>[2x]SNAMSAVMTPAGFTDYKVADITLAAWGRRELIIAESEMPALMGLRRKYAGQQPLKGAKILGCIHMTIQTGVLIETLVALGAEVRWSSCNIFSTQDQAAAAIAAAGIPVFAWKGETEEEYEWCIEQTILKDGQPWDANMVLDDGGDLTEILHKKYPQMLERIHGITEETTTGVHRLLDMLKNGTLKVPAINVNDSVTKSKNDNKYGCRHSLNDAIKRGTDHLLSGKQALVIGYGDVGKGSSQSLRQEGMIVKVAEVDPICAMQACMDGFEVVSPYKNGINDGTEASIDAALLGKIDLIVTTTGNVNVCDANMLKALKKRAVVCNIGHFDNEIDTAFMRKNWAWEEVKPQVHKIHRTGKDGFDAHNDDYLILLAEGRLVNLGNATGHPSRIMDGSFANQVLAQIHLFEQKYADLPAAEKAKRLSVEVLPKKLDEEVALEMVKGFGGVVTQLTPKQAEYIGVSVEGPFKPDTYRY

By hydrolyzing SAH to adenosine (Ado) and L-homocysteine (Hcy), the enzyme SAHase (SAH hydrolase) serves as an important regulator of SAM-dependent methylation through the control of the SAM:SAH ratio, and is an indicator of the biological methylation activity of the cell. SAHases are usually active as homotetramers. The protomer has a three-domain fold, with two prominent domains, the substrate- and cofactor-binding domains, separated by a deep crevice. A small C-terminal dimerization domain locks two subunits into a homodimer by quaternary complementation of the cofactor binding site, where a tightly but non-covalently bound nicotinamide adenine dinucleotide (NAD+) is found in its oxidized form.

Two complexes of Zn2+-containing PaSAHase were crystallized in the presence of K+ ions and adenosine (Ado/K+/Zn2+), or an inhibitor, 2′-deoxyadenosine (2′-dAdo/K+Zn2+). Additionally, the latter ligand as well as 3′-deoxyadenosine (non-metabolized adenosine analog) were used for crystallization of zinc-free enzyme in the presence of Rb+ (2′-dAdo/Rb+) or K+ (3′-dAdo/K+) cations. We present four crystal structures of PaSAHase/ligand/ion(s) complexes at resolutions of 1.35 to 1.75 Å. The complexes crystallize in two different forms, either as a tetramer or as a dimer from which the complete homotetramer is generated by crystallographic symmetry. In all presented PaSAHase complexes, the four subunits exist in the closed conformation and each of them binds an adenine nucleoside or adenine, as well as an alkali metal cation, K+ or Rb+, in the substrate binding area. The K+/Rb+ cations are bound in the monovalent cation coordinating loop (T380-S384) in close proximity of the purine ring of the ligand, but they do not interact with the ligand directly. The coordination sphere of the K+/Rb+ cations is a slightly distorted pentagonal bipyramid formed by two main-chain carbonyl oxygen atoms (T380 and H382) and the side-chain oxygen atoms of T380 and a highly conserved Q65 residue involved in ligand binding. Three water molecules complete the coordination sphere. Finally, the catalytic proficiency index kcat/Km is one to over two orders of magnitude higher in the presence of potassium than for other ions. These findings clearly demonstrate that the enzyme attains its maximum catalytic activity when the K+ cation is bound. The K+ ion stabilizes the enzyme-substrate complex in the closed conformation for a time interval required to complete the catalytic cycle.>[4x]GPGSMVVKDISLADWGRKELDIAETEMPGLMAAREEFGKSQPLKGARISGSLHMTIQTAVLIETLKVLGAEVRWASCNIFSTQDHAAAAIAATGTPVFAVKGETLEEYWTYTDQI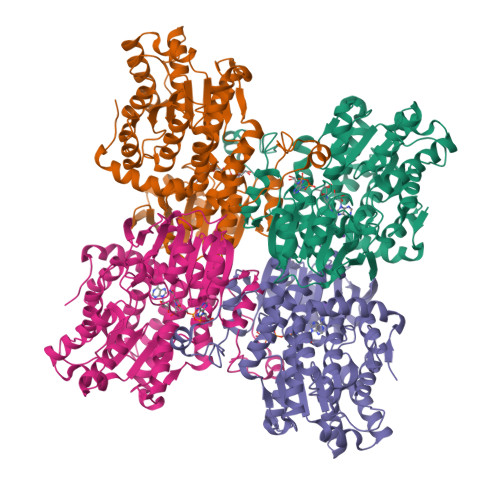FQWPDGEPSNMILDDGGDATMYILIGARAEAGEDVLSNPQSEEEEVLFAQIKKRMAATPGFFTKQRAAIKGVTEETTTGVNRLYQLQKKGLLPFPAINVNDSVTKSKFDNKYGCKESLVDGIRRGTDVMMAGKVAVVCGYGDVGKGSAQSLAGAGARVKVTEVDPICALQAAMDGFEVVTLDDAASTADIVVTTTGNKDVITIDHMRKMKDMCIVGNIGHFDNEIQVAALRNLKWTNVKPQVDLIEFPDGKRLILLSEGRLLNLGNATGHPSFVMSASFTNQVLGQIELFTRTDAYKNEVYVLPKHLDEKVARLHLDKLGAKLTVLSEEQAAYIGVTPQGPFKSEHYRY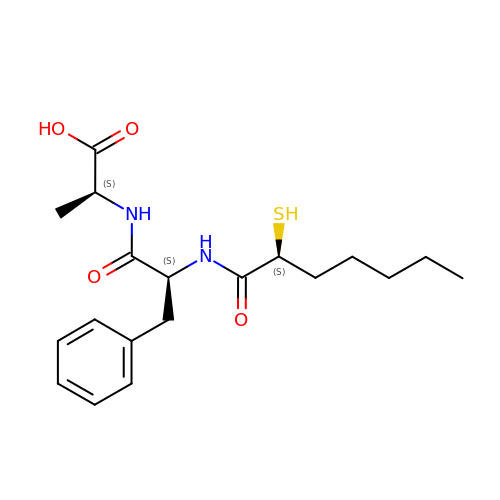[2(R,S)-2-SULFANYLHEPTANOYL]-PHE-ALA | C19 H28 N2 O4 S | GOIYKVXXGCPHQU-BPUTZDHNSA-N> MVSRFLIAEYRHLIENPSENFKISVNEKDMTEWDVILRGPPDTFYEGGLFKAKIAFPPEYPYAPPRLTFTSEMWHPNIYSDGKLCISILHGDNAEEQGMTWSPAQKIDTILLSVISLLNEPNPDSPANVDAAKSYRKLLYKEDLESYPMEVKRTVKKSLDECSPEDIEYFKNAA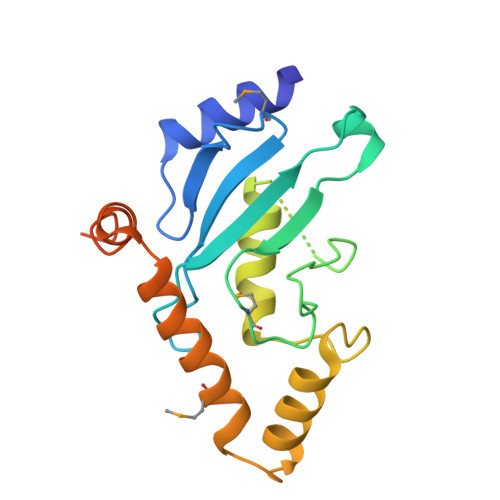SNVPPIPSDAYEDECHHHHHHHH>MDTTRFIRNFILFKDALQKQNFNNKDLNTTSMQAALQSEQLALSEESQYLQSEQVRAKMQIDFLGMQANLQNAKAETLNKLIQCQAMLKSLKDNAMINRANALVSLLQVQANAANGITTSNFEAAFKIIAQIGSEYNQITLNNGNVSVQEKEQTNELKTILNSLSKELEKLNQQSEVNSIQIFSDKLEVLKDAPARLWGFSTLSNAKEGFYNEANEQIASGSVCLFRSDKVRKHTITFKAINTKTSLSKNITISVIANKLKERMS[12x];>MDFTTLQNDFTNDYQKALIANNEFLE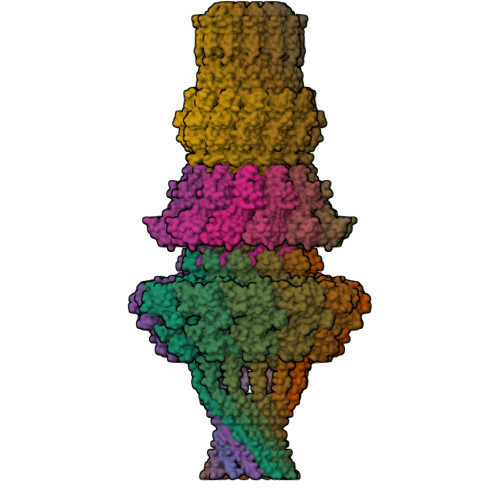AKKYYNGNQLPQDVLNIILERGQTPIIENMFKVIVNKILGYKIESISEIRLSPKQEEDRALSDLLNSLLQVFIQQENYDKSMIERDKNLLIGGLGVIQLWVSQDKDKNVEIEIKAIKPESFVIDYFSTDKNALDARRFHKMLEVSEQEALLLFGDSVIVNYSNVNHERIASVIESWYKEYNEETQSYEWNRYLWNRNTGIYKSEKKPFKNGACPFIVSKLYTDELNNYYGLFRDIKPMQDFINYAENRMGNMMGSFKAMFEEDAVVDVAEFVETMSLDNAIAKVRPNALKDHKIQFMNNQADLSALSQKAEQKRQLLRLLAGLNDESLGMAVNRQSGVAIAQRKESGLMGLQTFLKATDDMDRLIFRLAVSFICEYFTKEQVFKIVDKKLGDRYFKINSNDDNKIRPLKFDLILKSQLKTESRDEKWYNWNELLKILAPIRPDLVPSLVPLMLNDMDSPITNDVLEAIQNANALQQQNAEANAPYNQQIQALQIQKLQAEIMELQAKAHKYAEQGALSQTTNESEKINQAVAITEMQQQNANNANNEESNNKPKKKLKTSDKTTWRKYPSAQNLDY[12x];>MIEVSEVIAKVRERLNDNEVGNYEILDSVLVENINQALLKICLEFRLKKAITRSLITEEERFLTLNNLLGIESVKLDKKEIESRNTIEKDTGELELLILSDRISVTPFKIGELEVVYYTYEEIRNILETIKLPKICLDVLVYSVLCNLLEIPNNETNFSVLANYKQLLKLAKDNLTNYLSLMYSKNIHFSKVVRV[12x]>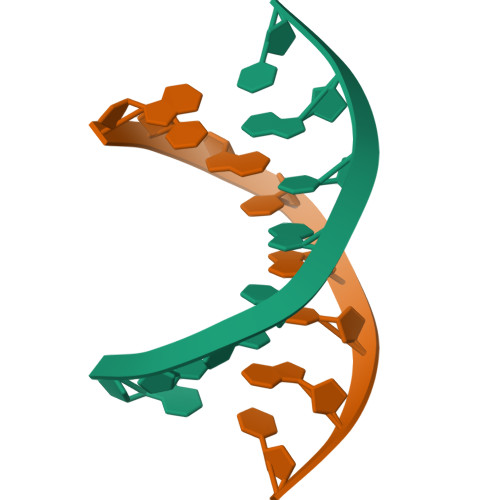 GTGCGCAC> ALLAEHLLRPLPADKQIETGPFLEAVSHLPPFFDCLGSPVFTPIKA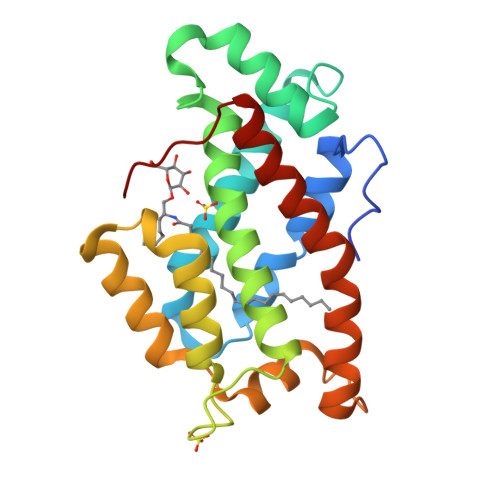DISGNITKIKAVYDTNPTKFRTLQNILEVEKEMYGAEWPKVGATLALMWLKRGLRFIQVFLQSICDGERDENHPNLIRVNATKAYEMALKKYHGWIVQKIFQAALYAAPYKSDFLKALSKGQNVTEEECLEKVRLFLVNYTATIDVIYEMYTRMNAELNYKV>[8x]PLVCLADFKAHAQKQLSKTSWDFIEGEADDGITYSENIAAFKRIRLRPRYLRDMSKVDTRTTIQGQEISAPICISPTAFHSIAWPDGEKSTARAAQEANICYVISSYASYSLED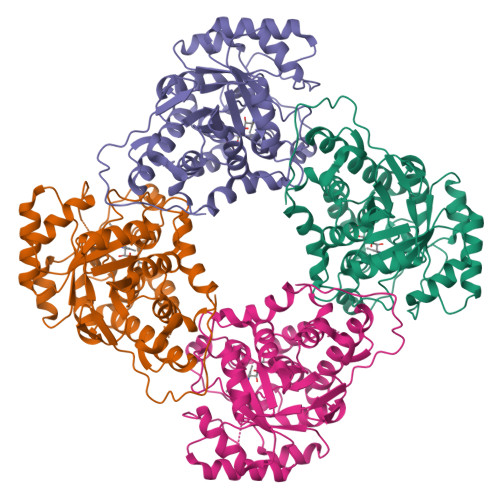IVAAAPEGFRWFQLYMKSDWDFNKQMVQRAEALGFKALVITIDTPVLGNRRRDKRNQLNLEANILLKDLRALKEEKPTQSVPVSFPKASFCWNDLSLLQSITRLPIILKGILTKEDAELAMKHNVQGIVVSNHGGRQLDEVSASIDALREVVAAVKGKIEVYMDGGVRTGTDVLKALALGARCIFLGRPILWGLACKGEDGVKEVLDILTAELHRCMTLSGCQSVAEISPDLIQFSRL>GSHGMRVIIA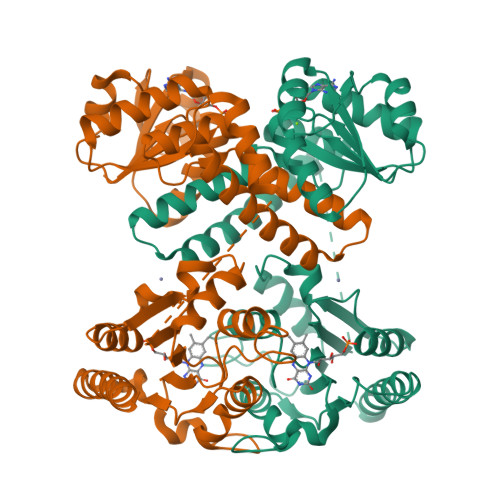GFGRFGQITGRLLLSSGVKMVVLDHDPDHIETLRKFGMKVFYGDATRMDLLESAGAAKAEVLINAIDDPQTNLQLTEMVKEHFPHLQIIARARDVDHYIRLRQAGVEKPERETFEGALKTGRLALESLGLGPYEARERADVFRRFNIQMVEEMAMVENDTKARAAVYKRTSAMLSEIITEDREHLSLIQRHGWQGTEEGKHTGNMADEPETKPSSTSGGLVPRGSSGMILIIYAHPYPHHSHANKRMLEQARTLEGVEIRSLYQLYPDFNIDIAAEQEALSRADLIVWQHPMQWYSIPPLLKLWIDKVFSHGWAYGHGGTALHGKHLLWAVTTGGGESHFEIGAHPGFDVLSQPLQATAIYCGLNWLPPFAMHCTFICDDETLEGQARHYKQRLLEWQEAHHG[2x]>MAHHHHHHVGTFENITAAPADPILGLADL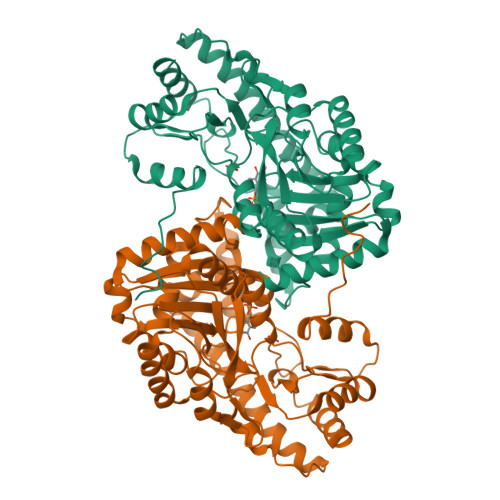FRADERPGKINLGIGVYFDETGKIPVLTSVKKAEQYLLENETTKTYLGIDGIPEFGRCTQELLFGKGSALINDKRARTAQTPGGTGALRVAADFLAKNTSVKRVWVSNPSWPNHKSVFNSAGLEVREYAYYDAENHTLDFDALINSLNEAQAGDVVLFHGCCHNPTGIDPTLEQWQTLAQLSVEKGWLPLFDFAYQGFARGLEEDAEGLRAFAAMHKELIVASSYSKNFGLYNERVGACTLVAADSETVDRAFSQMKAAIRANYSNPPAHGASVVATILSNDALRAIWEQELTDMRQRIQRMRQLFVNTLQEKGANRDFSFIIKQNGMFSFSGLTKEQVLRLREEFGVYAVASGRVNVAGMTPDNMAPLCEAIVAVL[2x]> TGLAADIRWTAYGVPHIRAKDERGLGYGIGYAYARDNACLLAEEIVTARGERARYFGSEGKSSAELDNLPSDIFYAWLNQPEALQAFWQAQTPAVRQLLEGYAAGFN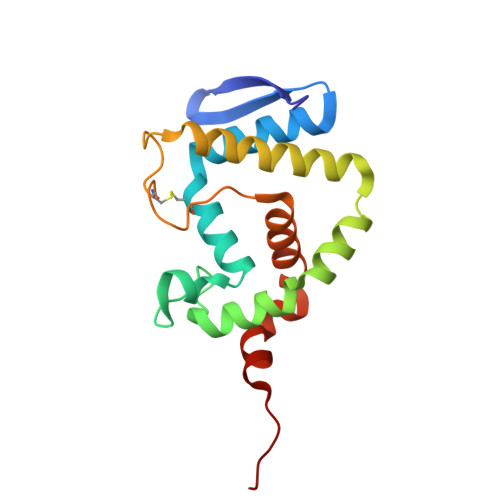RFLREADGKTTSCLGQPWLRAIATDDLLRLTRRLLVEGGVGQFADALVAAAPPGAE>[3x]MGRDPNSTNDTTTQNVVLTKYGFDKDVTAIDRATDQIWTGDGAKPLQGVDFTIYNVTANYWASPKDYKGSFDSAPVAATGTTNDKGQLTQALPIQSKDASGKTRAAVYLFHETNPRAGYNTSADFWLTLPAKAAADGNVYVYPKNVQKTTYERTFVKKDAETKEVLEGAGFKISNSDGKFLKLTDKDGQSVSIGEGFIDVLANNYRLTWVAESDATVFTSDKSGKFGLNGFADNTTTYTAV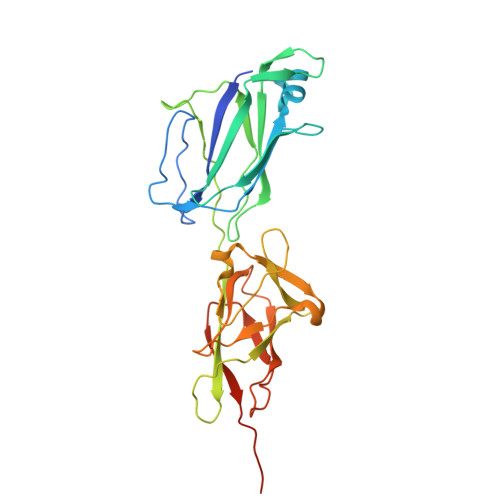ATNVPDGYDAAANTDFKADNSSSDILDAPSGILPLEHHHHHH>UGGAAGAAAUCGAAGAAGAUGAAGAACGCGAAGAAC[2x];>[2x]AUCUUCUUCGAUUUCUUCC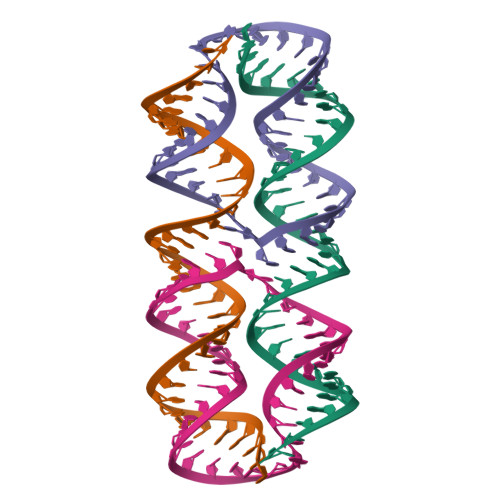AGUUCUUCGCGUUCUUC The PhoD family of extra-cytoplasmic phosphodiesterases are among the most commonly occurring bacterial phosphatases. The archetype of the family is Bacillus subtilis PhoD. This enzyme is a phosphodiesterase but also has significant phosphomonoesterase activity. The physiological role of PhoD is proposed to be the release of phosphate from cell wall teichoic acids under conditions of phosphate starvation.

The structure of PhoD was determined to a resolution of 2 Å via a multi-wavelength anomalous diffraction experiment using the iron cofactor as the source of the anomalous signal. The core of the PhoD structure is a sandwich of two long β-sheets flanked by α-helices of varying lengths. Three active site metal ions are coordinated by residues on loops on one face of the β-sandwich and are covered by a long C-terminal helix. With the knowledge that PhoD contains Fe3+ and Ca2+ ions (above) anomalous Fourier maps at three wavelengths allowed the assignment of the three active site metal ions as one Fe3+ ion and two Ca2+ ions, which we label CaA and CaB. At the Fe3+ site the sole difference in amino acid ligand sets between PhoD and the PAPs is a cysteine-for-aspartate substitution in PhoD (Cys-180). Specifically, the CaA site has irregular 8-fold coordination with all amino acid ligation being provide by Asp residues. The CaB ion has regular octahedral ligation with Asp and Asn ligands. The C-terminal region of the B. subtilis PhoD protein forms an α-helix (residues 560–577), which lies over the active site. The C-terminal helix blocks access to the catalytic site. The main chain crystallographic B-factor for the C-terminal helix is high (49.1 Å2) relative to the whole protein average (28.2 Å2), showing that the C-terminal helix is more mobile than the rest of the PhoD structure.

>APNFSSYPFTLGVASGDPLSDSVVLWTRLAPDPLNGGGMPKQAVPVKWEVAKDEHFRKIVRKGTEMAKPSLAHSVHVEADGLEPNKVYYYRFKTGHELSPVGKTKTLPAPGANVPQMTFAFASCQQYEHGYYTAYKHMAKEKLDLVFHLGDYIYEYGPNEYVSKTGNVRTHNSAEIITLQDYRNRHAQYRSDANLKAAHAAFPWVVTWDDHEVENNYANKIPEKGQSVEAFVLRRAAAYQAYYEHMPLRISSLPNGPDMQLYRHFTYGNLASFNVLDTRQYRDDQANNDGNKPPSDESRNPNRTLLGKEQEQWLFNNLGSSTAHWNVLAQQIFFAKWNFGTSASPIYSMDSWDGYPAQRERVINFIKSKNLNNVVVLTGDVHASWASNLHVDFEKTSSKIFGAEFVGTSITSGGNGADKRADTDQILKENPHIQFFNDYRGYVRCTVTPHQWKADYRVMPFVTEPGAAISTRASFVYQKDQTGLRKVSSTTIQGGVKQSDEVEEDRFFSHNKAHEKQMIKKRAKITN[2x]>AETVSFNFNSFSEGNPAINFQGDVTVLSNGNIQLTNLNKVNSVGRVLYAMPVRIWSSATGNVASFLTSFSFEMKDIKDYDPADGIIFFIAPEDTQIPAGSIGGGTLGVSDTKGAGHFVGVEFDTYSNSEYNDPPTDHVGIDVNSVDSVKTVPWNSVSGAVVKVTVIYDSSTKTLSVAVTNDNGDITTIAQVVDLKAKLPERVKFGFSASGSLGGRQIHLIRSWSFTS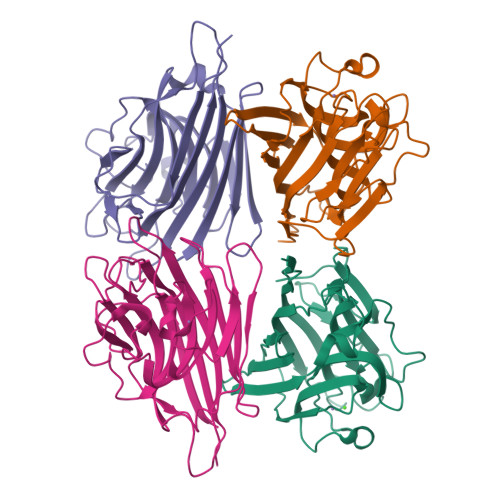TLITT[8x]> MIPGSFDYHRPKSIADAVALLTKLGEDARPLAGGHSLIPIMKTRLATPEHLVDLRDIGDLVGIRE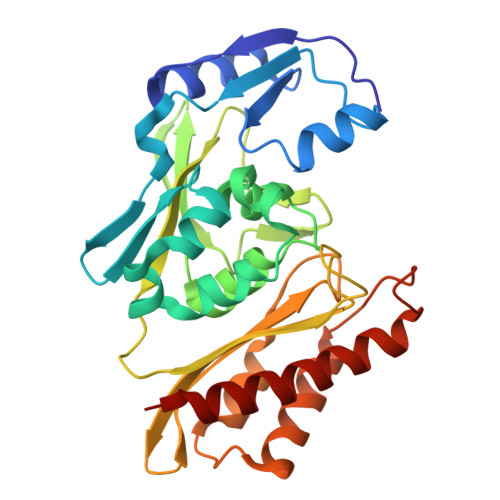EGTDVVIGAMTTQHALIGSDFLAAKLPIIRETSLLIADPQIRYMGTIGGNAANGDPGNDMPALMQCLGAAYELTGPEGARIVAARDYYQGAYFTAIEPGELLTAIRIPVPPTGHGYAYEKLKRKIGDYATAAAAVVLTMSGGKCVSASIGLTNVANTPLWAEEAGKVLVGTALDKPALDKAVALAEAITAPASDGRGPAEYRTKMAGVMLRRAVERAKARAKN(2~{S})-2-azanyl-5-[[(2~{R})-3-[(2~{R},5~{R})-5-(hydroxymethyl)-3,6-bis(oxidanylidene)-2-(phenylmethyl)-5-sulfanyl-piperazin-2-yl]sulfanyl-1-(2-hydroxy-2-oxoethylamino)-1-oxidanylidene-propan-2-yl]amino]-5-oxidanylidene-pentanoic acid | C22 H29 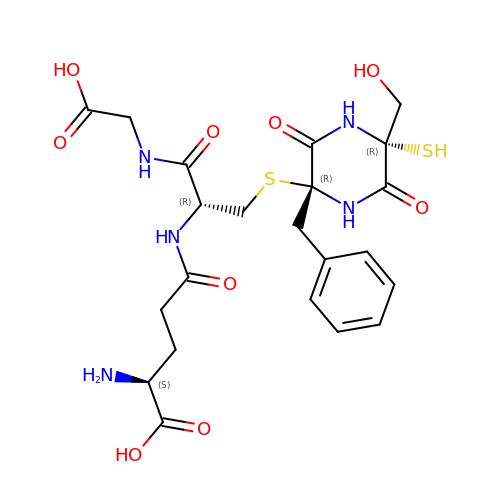N5 O9 S2 | BVLPJUGYSWKCGB-HCIHMXRSSA-N>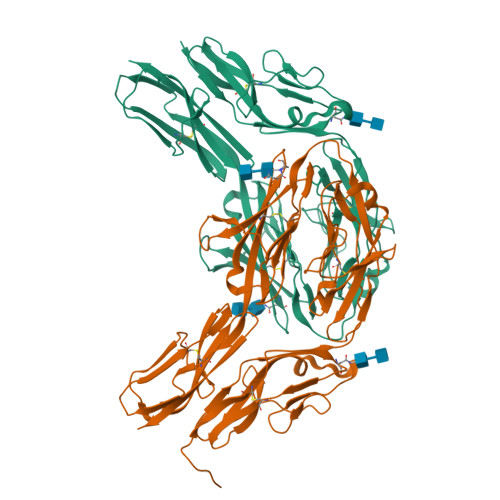[2x]AYFQGDQKGPVFLKEPTNRIDFSNSTGAEIECKASGNPMPEIIWIRSDGTAVGDVPGLRQISSDGKLVFPPFRAEDYRQEVHAQVYACLARNQFGSIISRDVHVRAVVAQYYEADVNKEHVIRGNSAVIKCLIPSFVADFVEVVSWHTDEEENYFPGAEYDGKYLVLPSGELHIREVGPEDGYKSYQCRTKHRLTGETRLSATKGRLVITEPISSSAPRTPALVQKPLELMVAHTISLLCPAQGFPAPSFRWYKFIEGTTRKQAVVLNDRVKQVSGTLIIKDAVVEDSGKYLCVVNNSVGGESVETVLTVTAPLSAKIDPPTQTVDFGRPAVFTCQYTGNPIKTVSWMKDGKAIGHSESVLRIESVKKEDKGMYQCFVRNDRESAEASAELKLG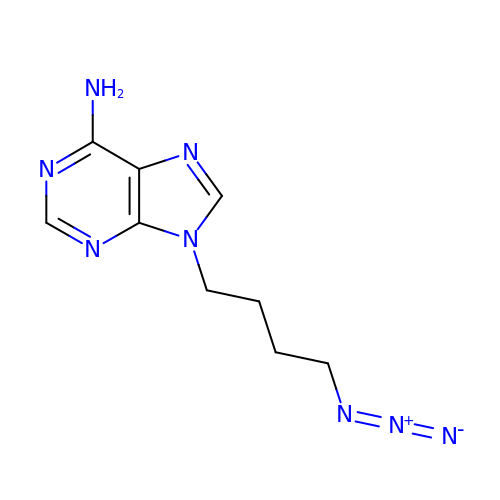9-(4-azidobutyl)purin-6-amine | C9 H12 N8 | HVEKFLZTZQALAB-UHFFFAOYSA-N3-(2-aminoquinazolin-6-yl)-1-(3,3-dimethylindolin-6-yl)-4-methylpyridin-2(1H)-one 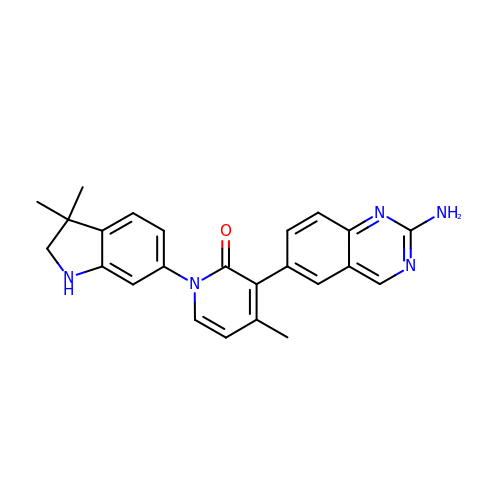| C24 H23 N5 O | LHLGUOHREUTYTO-UHFFFAOYSA-N>[2x]SNAMSMKKGNCKLHRMGEPHGPKVLLIHGAGFYWQTCFARIIRDLKDRYCLLIPELEGHTAHPREYMVSVEETAGKLGEALEELRVDKVQAIYGVSLGASVAVEMA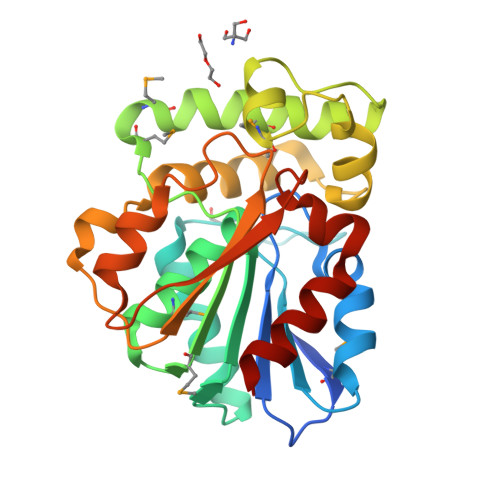IRGEIKVMNLLLDGGQYEGMGEMTEQYANIMADAFLNLLAGEHLPSPVKENMGFAANNDVEVLQPLIYEHITREALLHALLAAYRYDLKAKNARVDARVSVLIGGNEIYGAQFTPLLAEISRHPLDIYEFPNRGHAEVLSKEPEKISRLIREILNYC2-[(1~{R})-1-[2-azanyl-5-(1,3-dimethylpyrazol-4-yl)pyridin-3-yl]oxyethyl]-4-fluoranyl-~{N},~{N}-dimethyl-benzamide | C21 H24 F N5 O2 | 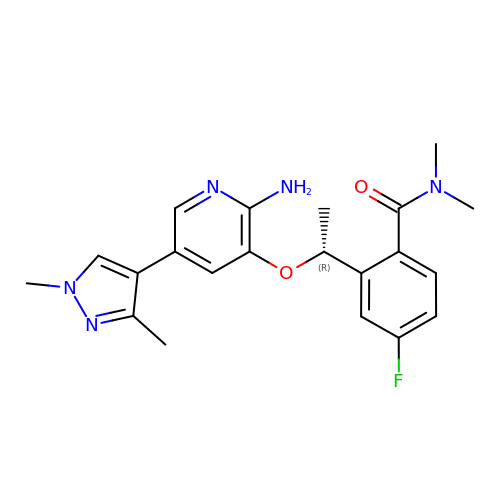CZKOZZRYDBLSRF-CYBMUJFWSA-N>RDRMVMGKIKRIEAGLPLTTAKGRTFGYDVIDTKLYINEEEAKQLRLIYDIFEEEQSITFLQKRLKKLGFKVRTYNRYNNWLTNDLYCGYVSYKDKVHVKGIHEPIISEEQFYRVQEIFSRMGKNPNMNKESASLLNNLVVCSKCGLGFVHRRKDTVSRGKKYHYRYYSCKTYKHTHELEKCGNKIWRADKLEELIIDRVNNYSFASRNI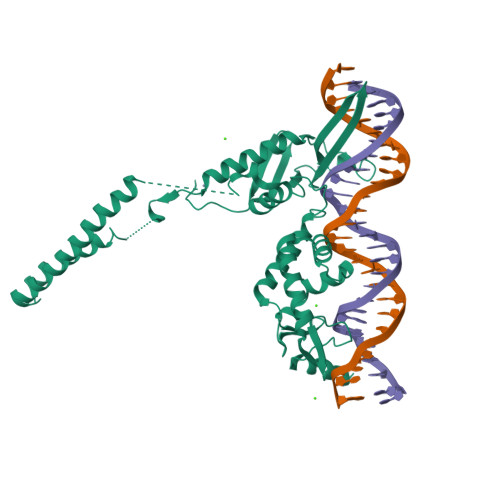DKEDELDSLNEKLKIEHAKKKRLFDLYINGSYEVSELDSMMNDIDAQINYYEAQIEANEELKKNKKIQENLADLATVDFNSLEFREKQLYLKSLINKIYIDGEQVTIEWLLEHHHHHH[4x]> MDIFREIASSMKGENVFISPPSISSVLTILYYGANGSTAEQLSKYVEKEADKNKDDISFKSMNKVYGRYSAVFKDSFLRKIGDNFQTVDFTDSRTVDAINKSVDIFTEGKINPLLDEPLSPDTSLLAISAVYFKAKWLMPFEKEFTSDYPFYVSPTEMVDVSMMSMYGEAFNHASVKESFGNFSIIELPYVGDTSMVVILPDNIDGLESIEQNLTDTNFKKWSDSMDAMFIDVHIPKFKVTGSYNLVDALVKLGLTE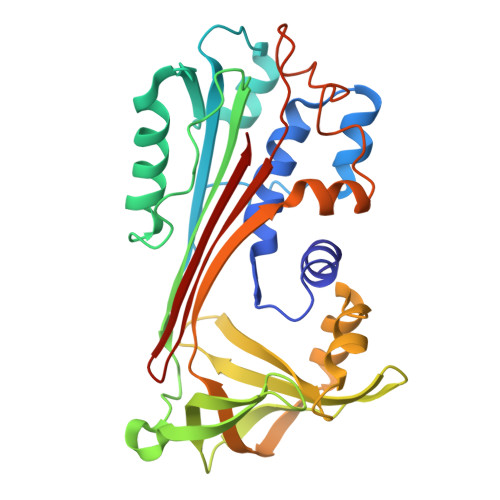VFGSTGDYSNMSNSDVSVDAMIHKTYIDVNEEYTEAAAATSAL>[2x]MTAHRSVLLVVHTGRDEATE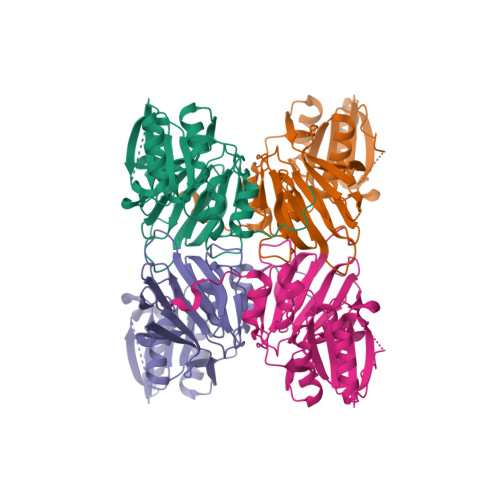TARRVEKVLGDNKIALRVLSAEAVDRGSLHLAPDDMRAMGVEIEVVDADQHAADGCELVLVLGGDGTFLRAAELARNASIPVLGVNLGRIGFLAEAEAEAIDAVLEHVVAQDYRVEDRLTLDVVVRQGGRIVNRGWALNEVSLEKGPRLGVLGVVVEIDGRPVSAFGCDGVLVSTPTGSTAYAFSAGGPVLWPDLEAILVVPNNAHALFGRPMVTSPEATIAIEIEADGHDALVFCDGRREMLIPAGSRLEVTRCVTSVKWARLDSAPFTDRLVRKFRLPVTGWRGK>MAQERPSCAVEPEHVQRLLLSSREAKKSAYCPYSRFPVGAALLTGDGRIFS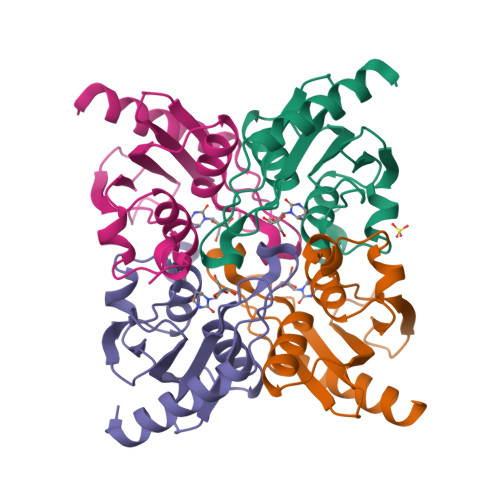GCNIENACYPLGVCAERTAIQKAISEGYKDFRAIAISSDLQEEFISPCGACRQVMREFGTDWAVYMTKPDGTFVVRTVQELLPASFGPEDLQKIQ[4x]>HMSSGNASWFQAIKAKKLNTPPPKFEGSGVPDNENIKPSQQHGYWRRQARFKPGKGGRCPVPDAWYFYYTGTGPAADLNWGDTQDGIVWVAAKGADTKSRSNQGTRDPDKFDQYPLRFSDGGPD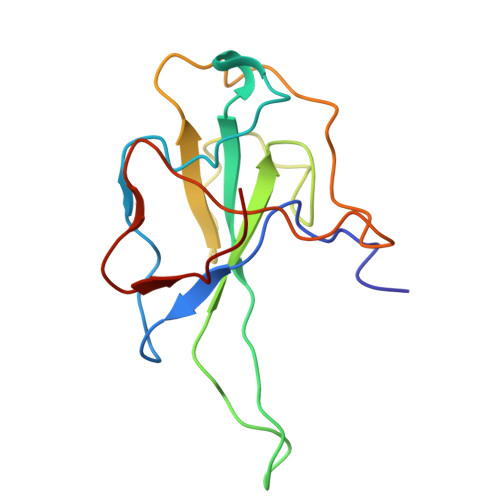GNFRWDFIPL[2x]> VAMVNTTTRLSDDALAFLSERHLAMLTTLRADNSPHVVAVGFTFDPKTHIARVITTGGSQKAVNADRSGLAVLSQVDGARWLSLEGRAAVNSDIDAVRDAELRYAQRYRTPRPNPRRVV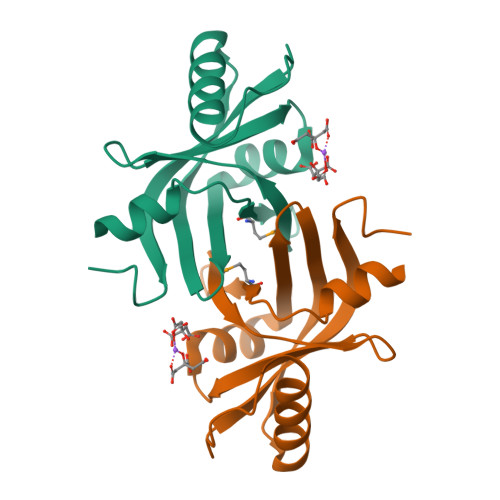IEVQIERVLGSADLLDRA>MIEGLSHMTFIVRDLERMTRILEGVFDAREVYASDTEQFS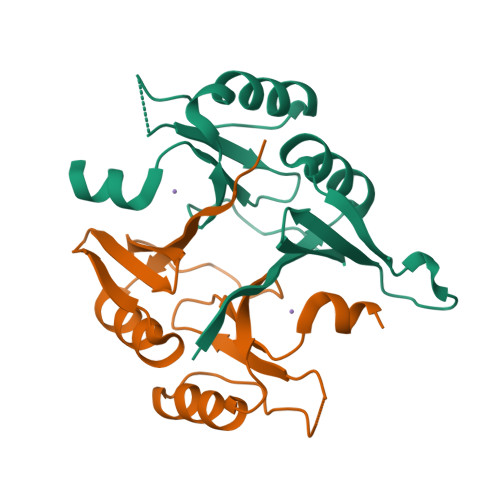LSREKFFLIGDIWVAIMQGEKLAERSYNHIAFKIDDADFDRYAERVGKLGLDMRPPRPRVEGEGRSIYFYDDDNHMFELHTGTLTERLARKAKGLEAAQ[2x]> RDEPPADGALKRAEELKTQANDYFKAKDYENAIKFYSQAIELNPSNAIYYGNRSLAYLRTECYGYALGDA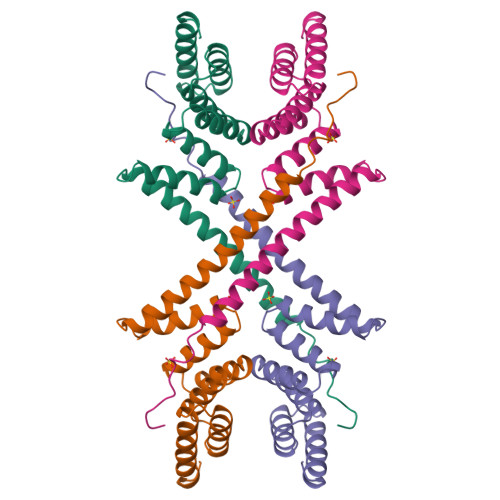TRAIELDKKYIKGYYRRAASNMALGKFRAALRDYETVVKVKPHDKDAKMKYQECNKIVKQKAFERAIAGDEHKRSVVDSLDIESMTIEDEYSGPKL Ubiquitin-specific protease 47 (USP47), a member of the USP family of deubiquitinating enzymes (DUBs), is involved in diverse cellular processes. USP47 is widely involved in tumor development, metastasis, and other processes while performing a more regulatory role in inflammatory responses, myocardial infarction, and neuronal development. The crystal structures of the catalytic domain, in its free and ubiquitin-bound states, reveal that the misaligned catalytic triads, ultimately, become aligned upon ubiquitin-binding, similar to USP7, thereby becoming ready for catalysis. Our study provides molecular details of USP47 regulation, substrate recognition, and the hotspots for drug discovery by targeting USP47.

We obtained crystals for cUSP47CD and determined the crystal structure at 2.6 Å resolution. The three molecules in an asymmetric unit have pairwise RMSD ≤ 0.65 Å for 316 Cα atoms. It revealed a canonical USP fold with three distinct subdomains: Thumb, Fingers, and Palm. The Fingers comprised four β strands in the center (β1, β2, β4, and β7), an α−helix (α7), and an additional two β strands (β5 and β6) at the tip that harbors four cysteine residues, which coordinates the structural Zn. In the apo form, the Sγ of the catalytic Cys97 was 10.0 Å from Nδ1 of His420 (insert), although the Nε2 of His420 made a hydrogen bond with Asn437 Oδ1. Therefore, the catalytic triads were incompetent for catalysis. In the free form, the His178 imidazole ring and the Trp169 indole ring form a π–π interaction, which hovers over a cluster of hydrophobic residues, e.g., Tyr98, Leu99, Ile139, Leu163, Phe167, Tyr175, Leu183, Leu186, and Met187 from α1, α5, and SL. The SL takes up a helical segment and puts the Tyr175 sidechain into the hydrophobic cluster. This couples with the rotation of the Tyr98 and the catalytic Cys97 away from the canonical active configuration. Arg309 in USP47 deserves special attention since it appears to stabilize BL1 conformation in the apo state, i.e., the guanidinium group of Arg309 stabilizes the switching loop by making H-bonds to His178, Asp179, Tyr175, and Tyr421 in all three molecules.

>[3x]MVRVEDSNGADTDTNPEGESSGYVRLAGNGLPGGEQQQASSSGVAAAPSVDSSPGRSVPLAIASSSSPANVANNQYAIPVDENGHRYVGLVNQAMTCYLNSLVQSLYMTPEFRNAMYDWEYVQQPAHIKEQRKKAEQSIPCQLQKLFLLLQTSENDSLETKDLTQSFGWTSNEAYDQHDVQELCRLMFDALEHKWKGTEHEKLIQDLYRGTMEDFVACLKCGRESVKTDYFLDLPLAVKPFGAIHAYKSVEEALTAFVQPELLDGSNQYMCENCKSKQDAHKGLRITQFPYLLTIQLKRFDFDYNTMHRIKLNDKMTFPDVLDLNDYVNKEKRSTTSSAWQQIGKNKSENEEDDMELGSPNPKRCTPGVQSPNRYQGSENVCVGQPIDHAAVDDIVKTSGDNVYELFSVMVHSGNAAGGHYFAYIKNLDQDRWYVFNDTRVDFATPLEIEKSFGGHPSGWNQSNTNAYMLMYRRIDPKRNARFILSNQLPQHIKDSQEKWKRLEREAE>VSLPVVLIADKLAPSTVAALGDQVEVRWVDGPDRDKLLAAVPEADALLVRSATTVDAEVLAAAPKLKIVARAGVGLDNVDVDAATARGVLVVNAPTSNIHSAAEHALALLLAASRQIPAADASLREHTWKRSSFSGTEIFGKTVGVVGLGRIGQLV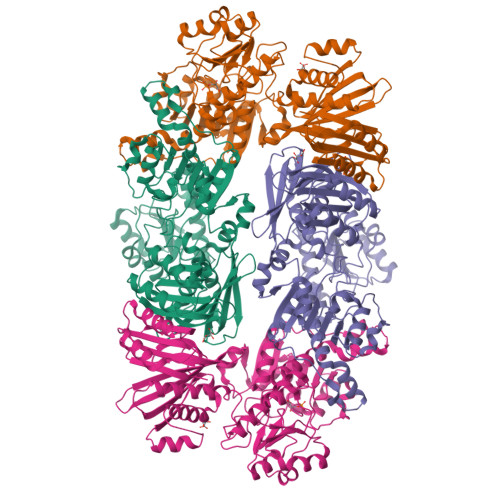AQRIAAFGAYVVAYDPYVSPARAAQLGIELLSLDDLLARADFISVHLPKTPETAGLIDKEALAKTKPGVIIVNAARGGLVDEAALADAITGGHVRAAGLDVFATEPCTDSPLFELAQVVVTPHLGASTAEAQDRAGTDVAESVRLALAGEFVPDAVNVGGGVVNEEVAPWLDLVRKLGVLAGVLSDELPVSLSVQVRGELAAEEVEVLRLSALRGLFSAVIEDAVTFVNAPALAAERGVTAEICKASESPNHRSVVDVRAVGADGSVVTVSGTLYGPQLSQKIVQINGRHFDLRAQGINLIIHYVDRPGALGKIGTLLGTAGVNIQAAQLSEDAEGPGATILLRLDQDVPDDVRTAIAAAVDAYKLEVVDLS[2x]> SMIRKQAESYANSTWEVLQYKDSGEPGVLEVFVTINGKVQNITFHIPKTIYMKFKSQTMPLQKIKNCLIEKSSASLPNNPKTSNPAGGQLFKITLPESVFLEEKENCTSIFNDENVLGVFEGTITPHQRAIMDLGASVTFRSKAMGALGKGIQQGFEMKDLSMAENERYLSGFSMDIGYLLHFPTSIGYEFFSLFKSWGDTITILVLKPSNQAQEINASSLGQIYKQMFEKKKGKIETYSYLVDIKEDINFEFVYFTDISKLYRRLSQETTKLKEERGLQFLLLLQSPFITKLLGTIRLLNQMPIVKLSLNEVLLPQLNWQPTLLKKLVNHVLSSGSWISHLIKLSQYSNIPICNLRLDSMDYIIDVLYARKLKKENIVLWWNEKAPLPDHGGIQNDFDLNTSWIMNDSEFPKINNSGVYDNVVLDVGVDNLTVNTILTSALINDAEGSDLVNNNMGIDDKDAVINSPSEFVHDAFSNDALNVLRGMLKEWWDEALKENSTADLLVNSLASWVQNPNAKLFDGLLRYHVHNLTKKALLQLVNEFSALGSTIVYADRNQILIKTNKYSPENCYAYSQYMMKAVRTNPMFSYLDLNIKRYWDLLIWMDKFNFSGLACIEIEEKENQDYTAVSQWQLKKFLSPIYQPEFEDWMMIILDSMLKTKQSYLKLNSGTQRPTQIVNVKKQDKEDSVENSLNGFSHLFSKPLMKRVKKLFKNQQEFILDPQYEADYVIPVLPGSHLNVKNPLLELVKSLCHVMLLSKSTILEIRTLRKELLKIFELREFAKVAEFKDPSLSLVVPDFLCEYCFFISDIDFCKAAPESIFSCVRCHKAFNQVLLQEHLIQKLRSDIESYLIQDLRCSRCHKVKRDYMSAHCPCAGAWEGTLPRESIVQKLNVFKQVAKYYGFDILLSCIADLT;> MFGSGNVLPVKIQPPLLRPLAYRVLSRKYGLSIKSDGLSALAEFVGTNIGANWRQGPATIKFLEQFAAVWKQQERGLFIDQSGVKEVIQEMKEREKVEWSHEHPIQHEENILGRTDDDENNSDDEMPIAADSSLQNVSLSSPMRQPTERDEYKQPFKPESSKALDWRDYFKVINASQQQRFSYNPHKMQFIFVPNKKQNGLGGIAGFLPDIEDKVQMFLTRYYLTNDRVMRNENFQNSDMFNPLSSMVSLQNELSNTNRQQQSSSNSITPIKNLLGRDAQNFLLLGLLNKNFKGNWSLEDPSGSVEIDISQTIPTQGHYYVPGCMVLVEGIYYSVGNKFHVTSMTLPPGERREITLETIGNLDLLGIHGISNNNFIARLDKDLKIRLHLLEKELTDHKFVILGANLFLDDLKIMTALSKILQKLNDDPPTLLIWQGSFTSVPVFASMSSRNISSSTQFKNNFDALATLLSRFDNLTENTTMIFIPGPNDLWGSMVSLGASGTLPQDPIPSAFTKKINKVCKNVVWSSNPTRIAYLSQEIVIFRDDLSGRFKRHRLEFPFNESEDVYTENDNMMSKDTDIVPIDELVKEPDQLPQKVQETRKLVKTILDQGHLSPFLDSLRPISWDLDHTLTLCPIPSTMVLCDTTSAQFDLTYNGCKVINPGSFIHNRRARYMEYVPSSKKTIQEEIYI

Hetero-tetrameric Pol epsilon plays a key role in replisome maturation and origin activation. Pol2 is the catalytic subunit, with the N-terminal half containing DNA synthesis/exonuclease functions. The C-terminal half of Pol2 (C-Pol2) has been predicted to contain a second polymerase fold, which has become inactivated during evolution, and is followed by a zinc-finger appendix. Notably, the catalytic domain of Pol epsilon is dispensable for viability (though cells are sick), while the non-catalytic C-Pol2 is essential.

To understand the role of the essential Pol epsilon modules during DNA replication, we studied the structure of a truncation mutant of the yeast tetrameric complex, lacking the dispensable, flexibly tethered N-terminal catalytic domain of Pol2 (hereafter, deltacat). To mitigate this problem, we incubated our preparation with 0.01% of crosslinking agent glutaraldehyde for one minute on ice, before cryo-grid making. We determined a 3D structure of the deltacat core based on 161,372 particles, to an average resolution of 4.45 Å (4.3 Å in the core and 5 Å in the periphery), revealing a compact assembly of dimensions 100 × 90 × 60 Å. To interpret the map, we have docked a recently published structure of human C-terminal Dpb2 bound to the Pol2 C-terminal zinc-finger appendix, providing an unambiguous fit. Docking of a Pol1-based homology model of C-Pol2 into the cryo-EM density required splitting the polymerase into three domains, which were used in independent rigid-body fitting and subsequent real-space refinement. The resulting structure shows a polymerase fold with jaws spread wide open. In agreement with the notion that certain elements are only flexibly tethered to the deltacat core, no density was retrieved for the N-terminal domain of Dpb2, nor for the histone-like subunits Dpb3-Dpb4. For example, the C-terminus of Dpb2 intimately contacts C-Pol2, explaining why a truncation of the last six amino acids in Dpb2 prevents Dpb2 binding to Pol2-Dpb3-Dpb4 and results in a lethal phenotype. Likewise, a so-called ZnF1 element in the Pol2 zinc-finger appendix emerges as the organizing center of the deltacat core, explaining why cysteine-to-alanine single amino acid changes in this region can alter the essential non-catalytic Pol epsilon core, hence abolishing cellular growth. Furthermore, inspecting a more complete Pol2 structure that extends beyond the conserved polymerase module revealed that the C-terminal zinc-finger appendix occludes the DNA-binding groove in the dead polymerase fold.> MTSRKKVLLKVIILGDSGVGKTSLMNQYVNKKFSNQYKATIGADFLTKEVMVDDRLVTMQIWDTAGQERFQSLGVAFYRGADCCVLVFDVTAPNTFKTLDSWRDEFLIQASPRDPENFPFVVLGNKIDLENRQVATKRAQAWCYSKNNIPYFETSAKEAI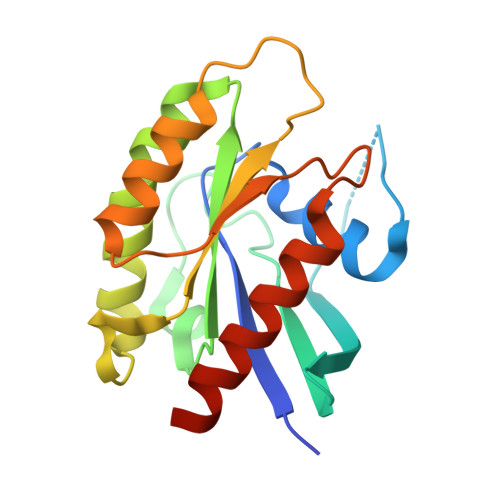NVEQAFQTIARNALKQETEVELYNE> MKSVITTVVSAADAAGRFPSNSDLESIQGNIQRSAARLEAAEKLAG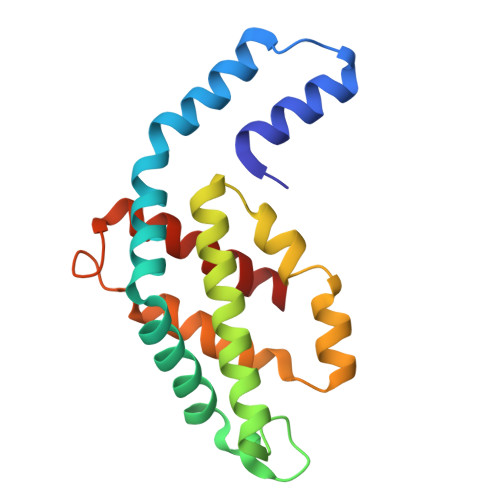NHEAVVKEAGDACFAKYAYLKNPGEAGENQEKINKCYRDVDHYMRLVNYCLVVGGTGPLDEWGIAGAREVYRTLNLPTSAYVASIAYTRDRLCVPRDMSAQAGVEFSAYLDYLINALS(3R,4R,5R)-3-hydroxy-5-(hydroxymethyl)piperidin-4-yl beta-D-glucopyranoside 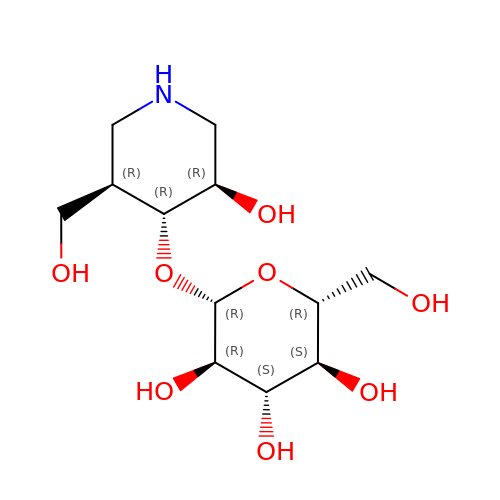| C12 H23 N O8 | LEOSSOWHBSKZSO-WUYFHPBOSA-N>[6x]MYLPDDSPAKRLLFQMVGNAINRNTQQLTQDLRAMPNWSLRFVYIVDRNNQDLLKRPLPPGIMV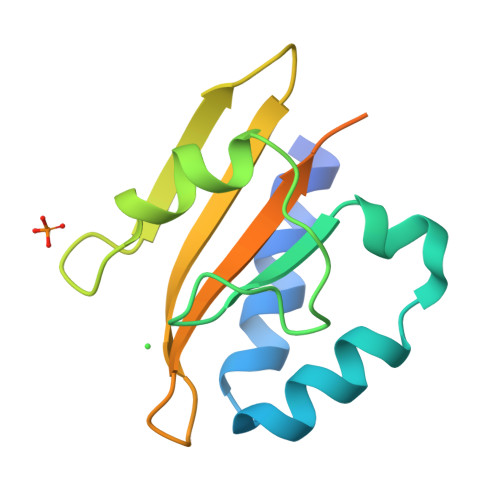LAPRLTAKHPYDKVQDRNRKLYGRHITLNDGNSVKVVTISAGRDEGPDRDIIWEMFLENLEHHHHHH5-[(Z)-(aminomethylidene)amino]-1-(5-O-phosphono-beta-D-ribofuranosyl)-1H-imidazole-4-carboxylic 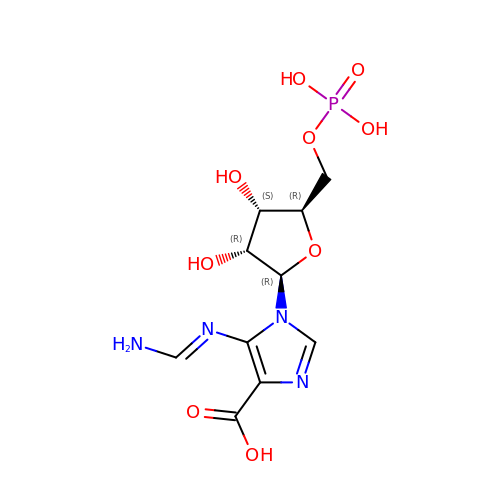acid | C10 H15 N4 O9 P | CEVAZLJDKSQTJT-FJGDRVTGSA-N>KDSAPRKPAEEPSPSVGEARPEPAKAEEKPAEPVSRPTKVVKTPVRGGMQIYAAGGDLIVLAAVSPGAELLADGNIHVYGPMRGRALAGVKGDATARIFCQQLAAELVSIAGNYKVAEDLRRSPQWGKAVHVSLSGDVLNITRL[11x];>[11x]MAKILVVTSGKGGVGKTTTSAAIGTGLALRGFKTVIVDFDVGLRNLDLIMGCERRVVYDFVNVVNGEATLTQALIKDKRLE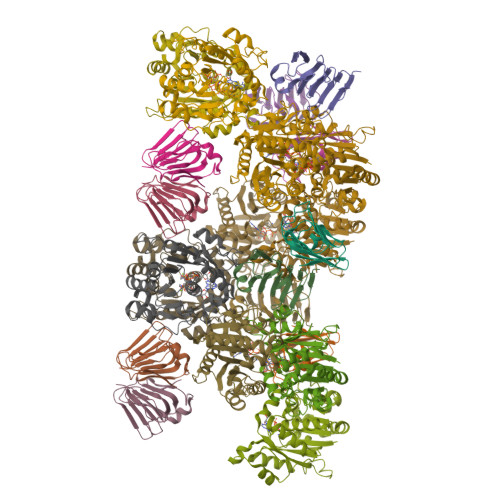NLHVLAASQTRDKDALTKEGVEKVMAELRKDFEYIICDSPAGIEKGAHLAMYFADEAIVVTNPEVSSVRDSDRMLGLLASKSQRAEKGEEPIKEHLLLTRYNPERVTKGEMLSVDDVEEILAIRLLGVIPESQAVLKASNQGVPVILDEQSDAGQAYSDAVDRLLGKEIPHRFLDVQKKGFLQRLFGGRE> TGAEPQALPSDPLEQALHQAWQAQLGAPPRAGQGFYAAGGDSLRAVHLLATLRQRLSRRVPLQAFAGGPATPEALLELLRQAAPEGDEPEPSAGAAGLSLAERRLWVAQQLAPEDTSYNLLAHLRIVGATADAIEQALRQLLERHVALRRRVETGVDGPQPHALAAHAVPLQRLLASDAVHAERLLEDGVRREGARVFDLAHEAPARLLLVVTRDSARADLLLSVHHYAFDDVSLAVFAAELKTLLDGGRLGVLASTPEQVAARERAALASGRLDRVAERWAERLLPLAKAPGAAPARPEESGGRAGQRLALPVSAAVHAACRALAERTSVSPFSAALQAFAEVLGAELGVDDLLVGVALAGRSRLEMQGLVGCFVNLLPLAVGLRPEQSVEWRLRQVGHDLLELLEHQDVPLECVTQALRQRGASGLPIRIACGAHNGRAAPAVDAGVRVEADFIPVPGARLDLTLWLEDQPQGWLAVWTGVSAIFDLHRIERLHQAWERRLLANAGEPISKRMSPEGCNAS

Non-ribosomal peptide synthetases (NRPS) are multi-modular/domain enzymes that catalyze the synthesis of bioactive peptides. A crucial step in the process is peptide elongation accomplished by the condensation (C) domain with the aid of a peptidyl carrier or thiolation (T) domain. Here, we examined condensation reaction carried out by NRPS AmbB involved in biosynthesis of l-2-amino-4-methoxy-trans-3-butenoic acid (AMB) in P. aeruginosa. We determined crystal structures of the truncated T–C bidomain of AmbB in three forms, the apo enzyme with disordered T domain, the holo form with serine linked phosphopantetheine (Ppant) and a holo form with substrate (l-alanine) loaded onto Ppant.

Crystal structure of the apo form of AmbB T-C (residues 727–1249) was determined at a resolution of 2.4 Å. There is one molecule per asymmetric unit. The structure revealed a typical V-shaped condensation domain consisting of two subdomains, namely an N-terminal lobe (Gly824–Ser997) and a C-terminal lobe (Gly998–Ala1233) subdomains. The active site of the C domain is at the central groove formed by the two subdomains and has a conserved HHxxxD motif in a loop between strand β6 and helix α4. There was no visible electron density for the T domain. This is likely due to inherent flexibility of the T domain as well as the absence of the cofactor, phosphopantetheine (Ppant). Residues constituting the loop region in the C domain, Gly881–Gly884, Lys1016–Arg1030, Asn1165–Asp1172 and Pro1198–Glu1200 are disordered and not built into the structure. A detergent molecule from the crystallization condition, MEGA-9 is bound to the peripheral side of the C terminal subdomain between helix α8 and helix α11. Such a binding mode far away from the active site is likely to be a crystallization artefact with no functional role. The C domain of apo and holo AmbB T–C show a quasi-identical conformation suggesting that it does not undergo obvious conformation change upon Ppant binding, at least by its upstream T domain.> MQQGQMAYDRAITVFSPDGRLFQVEYAREAVKKGSTALGMKFANGVLLISDKKVRSRLIEQNSIEKIQLIDDYV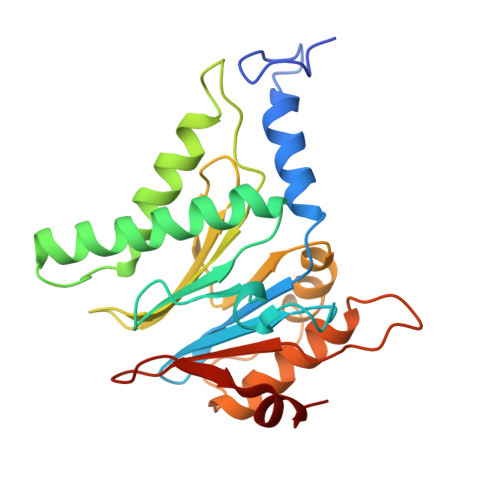AAVTSGLVADARVLVDFARISAQQEKVTYGSLVNIENLVKRVADQMQQYTQYGGVRPYGVSLIFAGIDQIGPRLFDCDPAGTINEYKATAIGSGKDAVVSFLEREYKENLPEKEAVTLGIKALKSSLEEGEELKAPEIASITVGNKYRIYDQEEVKKFL> TSWRSEATFQFTVER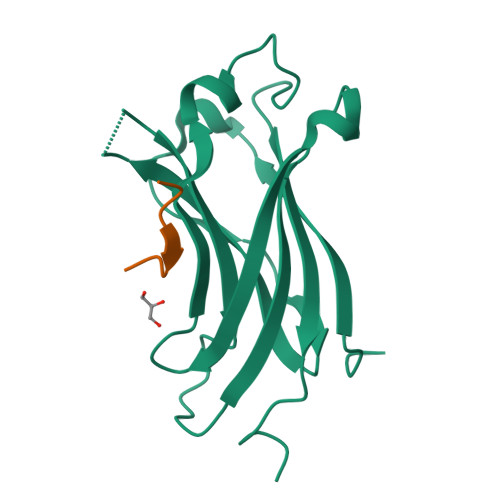FSRLSESVLSPPCFVRNLPWKIMVMPRFYPDRPHQKSVGFFLQCNAESDSTSWSCHAQAVLKIINYRDDEKSFSRRISHLFFHKENDWGFSNFMAWSEVTDPEKGFIDDDKVTFEVFVQADAPHGVAW;> SPGEGPSG> HHAADYVLYKDATKPVEDRVADLLGRMTLAEKIGQMTQIERLVATPDVLRDNFIGSLLSGGGSVPRKGAT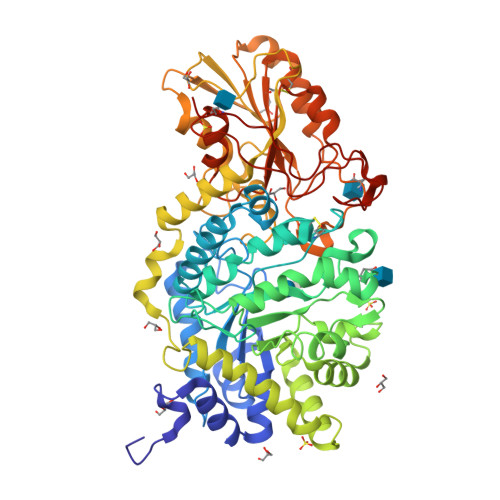AKEWQDMVDGFQKACMSTRLGIPMIYGIDAVHGQNNVYGATIFPHNVGLGATRDPYLVKRIGEATALEVRATGIQYAFAPCIAVCRDPRWGACYASYSEDRRIVQSMTELIPGLQGDVPKDFTSGMPFVAGKNKVAACAKHFVGDGGTVDGINENNTIINREGLMNIHMPAYKNAMDKGVSTVMISYSSWNGVKMHANQDLVTGYLKDTLKFKGFVISDWEGIDRITTPAGSDYSYSVKASILAGLDMIMVPNKYQQFISILTGHVNGGVIPMSRIDDAVTRILRVKFTMGLFENPYADPAMAEQLGKQEHRDLAREAARKSLVLLKNGKTSTDAPLLPLPKKAPKILVAGSHADNLGYQCGGWTIEWQGDTGRTTVGTTILEAVKAAVDPSTVVVFAENPDAEFVKSGGFSYAIVAVGEHPYTETKGDNLNLTIPEPGLSTVQAVCGGVRCATVLISGRPVVVQPLLAASDALVAAWLPGSEGQGVTDALFGDFGFTGRLPRTWFKSVDQLPMNVGDAHYDPLFRLGYGLTTNATKKY N-[(2Z,3R,4R,5S,6R)-4,5-dihydroxy-6-(hydroxymethyl)-2-{[(phenylcarbamoyl)oxy]imino}tetrahydro-2H-pyran-3-yl]-2-ethylbutanamide | C19 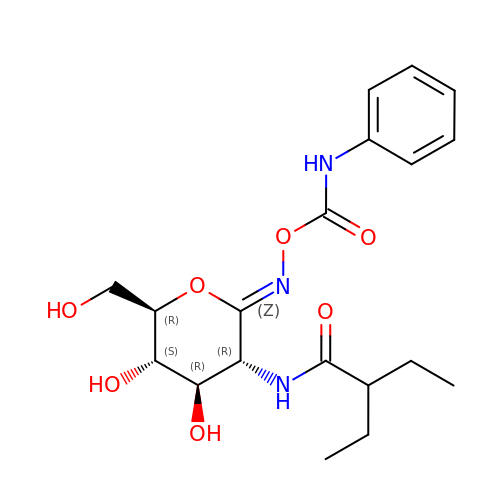H27 N3 O7 | ILCJHDDOBKGXME-OXSJTRRESA-N>[3x]NDDKEAKK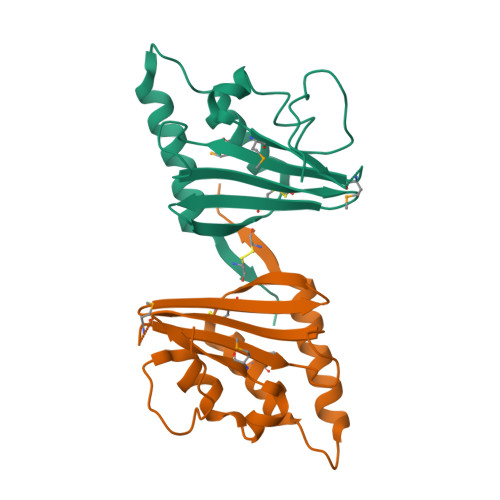EAQEKEKNTPNGLVYTNLDFDSFKATIKNLKDKKVTFKEVNPDIIKDEVFDFVIVNRVLKKIKDLKHYDPMIEKIFDEKGKEMGLNVEIQINPEVKDFFTFKSISTTNKQRCFLSLRGETREILCDNKLYNMLLAVFNSYDPNDLLKHISTVESLKKIFYTITCEAVY>GSMTTFRIENVRIETINDFDMVKFDLVTDLGRVELAEHVNYDSE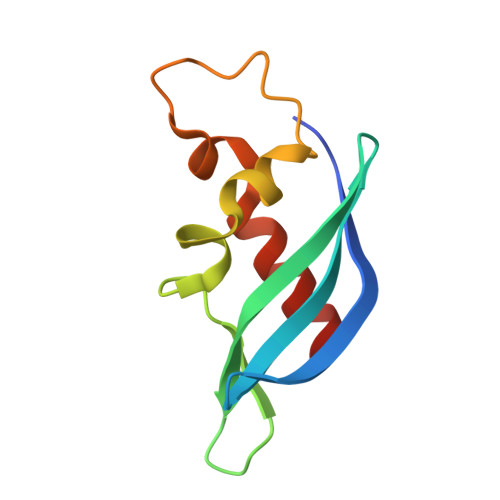GDFKSVEYTDSNIRYNMVDELCSVFDLTDKPSLMPAIDYVTFAEIIEAVEEMLEA[3x]>[2x]NVDEFLFISNNFKQYKEFI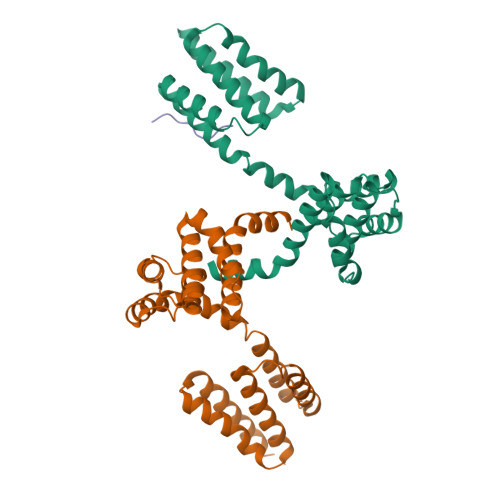DMDTAKHYFECRNIEGLNHILDSYKDSKSTKEKNLFALVKVLLATLTEEDCLTERTYLSNYLINIETWSHYETVLFNNCMFIFESCFIEMVFSKVILNLDKYNTLRYYGNESIRMFVNMLILFIQRQEYDKASEILAKIEDYQLNDDCLYERCCVSFFDGIIGLINGKEGAEQKCVQILEIFQLLNCKTIHHMFQTYLEAIKHKLSLEHHHHHH;> MWLLLLFL>SPLAAYEVDDSTGYLTSDVGGPIQDQTSLKAGIRGPTLLEDFMFRQKIQHFDHERVPERAVHARGAGAHGTFTSYADWSNITAASFLNATGKQTPVFVRFSTVAGSRGSADTARDVHGFATRFYTDEGNFDIVGNNIPVFFIQDAIQFPDLIHSVKPRPDNEIPQAATAHDSAWDFFSQQPSTMHTLFWAMSGHGIPRSYRHMDGFGVHTFRFVKDDGSSKLIKWHFKSRQGKASLVWEEAQVLSGKNADFHRQDLWDAIESGNGPEWDVCVQIVDESQAQAFGFDLLDPTKIIPEEYAPLTKLGLLKLDRNPTNYFAETEQVMFQPGHIVRGIDFTEDPLLQGRLFSYLDTQLNRNGGPNFEQLPINMPRVPIHNNNRDGAGQMFIHRNKYPYTPNTLNSGYPRQANQNAGRGFFTAPGRTASGALVREVSPTFNDHWSQPRLFFNSLTPVEQQFLVNAMRFEISLVKSEEVKKNVLTQLNRVSHDVAVRVAAAIGLGAPDADDTYYHNNKTAGWSIVGSGPLPTIKTLRVGILATTSESSALDQAAQLRTRLEKDGLVVTVVAETLREGVDQTYSTADATGFDGVVVVDGAAALFASTASSPLFPTGRPLQIFVDAYRWGKPVGVCGGKSSEVLDAADVPEDGDGVYSEESVDMFVEEFEKGLATFRFTDRFALDS[4x]

Catalases (hydrogen-peroxide:hydrogen-peroxide oxido­reductases; EC 1.11.1.6) are redox enzymes that are responsible for the dismutation of hydrogen peroxide into water and molecular oxygen. The structures reveal a homotetrameric enzyme in which each of the four active sites consists of a pentacoordinated iron protoporphyrin IX prosthetic group with a tyrosin­ate axial ligand. The heme is deeply buried inside the protein, with a complex network of channels providing access to the exterior. We have previously shown that in addition to catalase activity, the catalase from S. thermophilum (CATPO) possesses a promiscuous phenolic oxidase activity in the absence of hydrogen peroxide.

We therefore generated a series of site-directed mutants around the putative 3TR/catechol binding pocket to further test this hypothesis. The residues Pro158, His246, Gln293, Ile313, Ile314, Glu316, Leu321 and Val536 surround the 3TR binding pocket and are structurally homologous to the residues that bind NADPH in the mammalian catalases. Specifically, the variants P158W, H246W, Q293W, I313F, I314F, E316F, E316H, L321A, V536A and V536W were constructed. The catechol oxidase activities of the H246W, I314F, L321A and V536W variants were noticeably reduced (50–92%) with respect to the wild-type enzyme, whereas the E316F, E316H, I313F and V536A variants of CATPO had little effect on the oxidase activity. However, CATPO contains a C-terminal extension, residues 533–537, that does not exist in the NADPH-binding catalases and that lies across the upper region of this pocket, preventing the binding of NADPH. Val536 is part of the C-terminal extension of CATPO that blocks the upper part of the NADPH-binding pocket in mammalian catalases and thus it was surprising that changes in this residue had such marked effects on the catalase activity.>[2x]MSLEDRKNERLPSDLARRATAIIEMPDGVLVTASRGGRYNLPGGKANRGELRSQALIREIREETGLRINSMLYLFDHITPFNAHKVY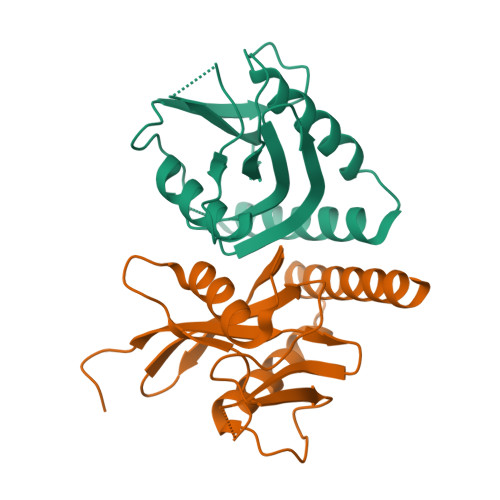LCIAQGQPKPQNEIERIALVSSPDTDMDLFVEGRAILRRYARLRNEETAKGEALRALLGLARYIAKVDEGHHHHHH>GSKVMQKDVLAQLMEHLETGQYKKREKTLAYMTKILEQGIHEYYKSFDNDTARKMALDYFKRINDDKGMIYMVVVDKNGVVLFDPVNPKTVGQSGLDAQSVDGVYYVRGYLEAAKKGGGYTYYKMPKYDGGVPEKKFAYSHYDEVSQMVIAATSYYTDINTENKAIKEGVNKVFNENTTR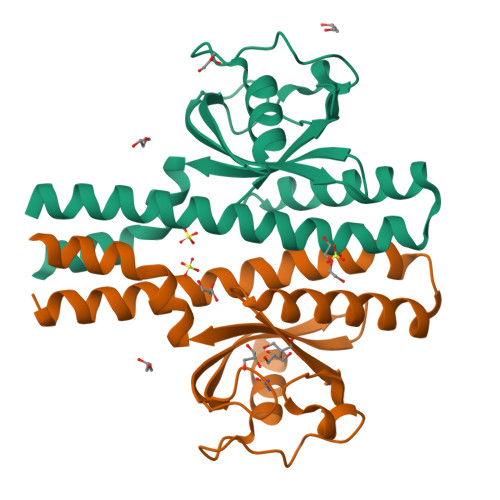L[2x]> FRAIIESPEGAGHVGYQYRRNTGSTMRMVSDVLDERVSLWDFHCDPSGNVIQPGPNVDSRQYLQAAIDYVSSNGGGTITIPAGYTWYLGSYGVGGIAGHSGIIQLRSNVNLNIEGRIHLSPFFDLKPFQVFVGFDNGDPASSGNLENCHIYGHGVVDFGGYEFG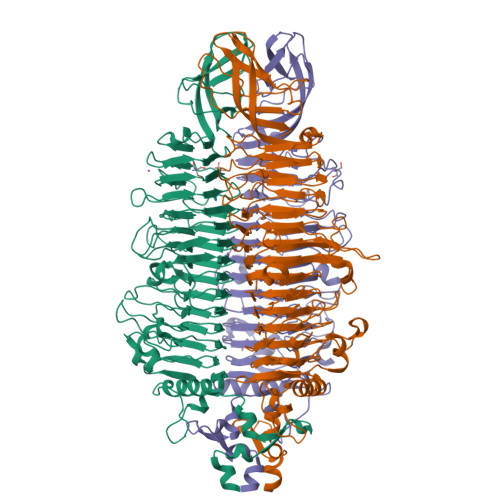ASSQLRNGVAFGRSYNCSVTGITFQNGDVTWAITLGWNGYGSNCYVRKCRFINLVNSSVNANHSTVYVNCPYSGVESCYFSMSSSFARNIACSVELHQHDTFYRGSTVNGYCRGAYVVMHAAEAAGAGSYAYNMQVENNIAVIYGQFVILGSDVTATVSGHLNDVIVSGNIVSIGERAAFSAPFGAFIDIGPDNSGASNVQDIQRVLVTGNSFYAPANITDSAAITLRANLNGCTFIANNFDCRYMVYNAPGTTSPVVQNLVWDKSNVIGGTHANQRAGQNLFDMQFASVVNSTIEVQLSCEDLSMFSCILFPASCQLSYSKITVDSAWTKSMSNTAVFEGNQQAGANVYVSYPATVNLTSYNTQGAVPFFSTDTNYAWVTSAYSLSINENLDFSPPATYTNKANGQLVGVGYNEIGGVRSVSVRLMLQRQV>GSHMPKMEVFQEYYGIPPPPGAFGPFLRLNPGDIVELTKAEAEHNWWEGRNTATNEVGWFPCNRVHPYV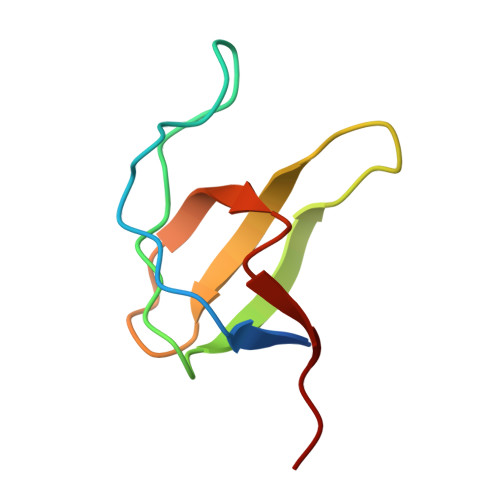H[4x]4-(2-azanyl-8-methoxy-quinazolin-6-yl)phenol | 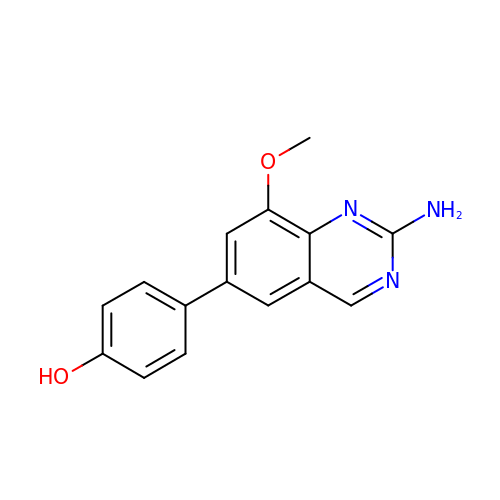C15 H13 N3 O2 | XMZXPVWZSUCWOA-UHFFFAOYSA-N>MFNSLLSGTTTPNSGRASPPASEMPIDNDHVAVARPAPRRRRIVVAMTGATGAMLGIKVLIALRRLNVETHLVMSKWAEATIKYETDYHPSNVRALADYVHNINDMAAPVSSGSFRADGMIVVPCSMKTLAAIHSGFCDDL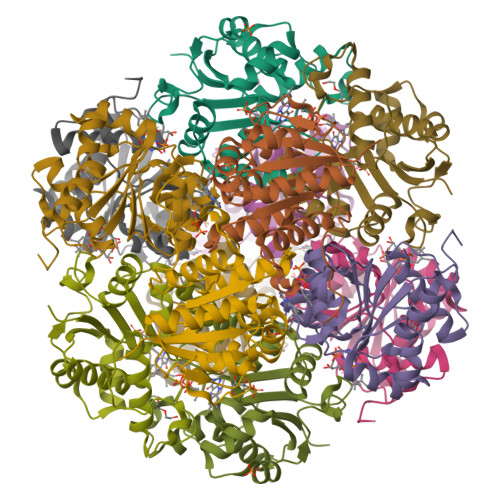ISRTADVMLKERRRLVLVARETPLSEIHLRNMLEVTRAGAVIFPPVPAFYIKAGSIEDLIDQSVGRMLDLFDLDTGDFERWNGWEK[6x]> SMKQTGYLTIGGQRYQAEINDLENLGEMGSGTCGQVWKMRFRKTGHVIAVKQMRRSGNKEENKRILMDLDVVLKSHDCPYIVQCFGTFITNTDVFIAMELMGTCAEKLKKRMQGPIPERILGKMTVAIVKALYYLKEK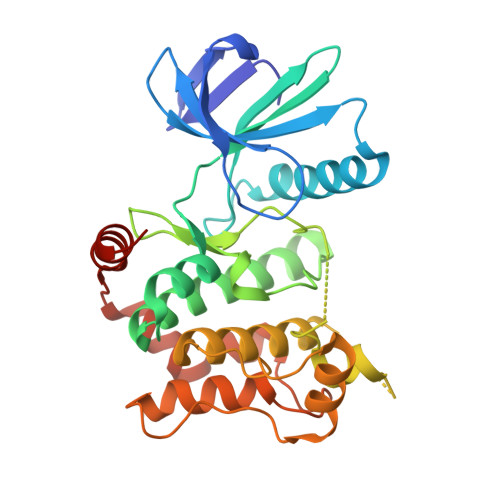HGVIHRDVKPSNILLDERGQIKLCDFGISGRLVDDKAKDRSAGCAAYMAPERIDPPDPTKPDYDIRADVWSLGISLVELATGQFPYKNCKTDFEVLTKVLQEEPPLLPGHMGFSGDFQSFVKDCLTKDHRKRPKYNKLLEHSFIKRYETLEVDVASWFKDVMAKTESPR> MSVNSIYTDREEIDSEFEDEDFEKEGIATVERAMENNHDLDTALLELNTLRMSMNVTYHEVRIATITALLRRVYHFIATQTLGPKDAVVKVFNQW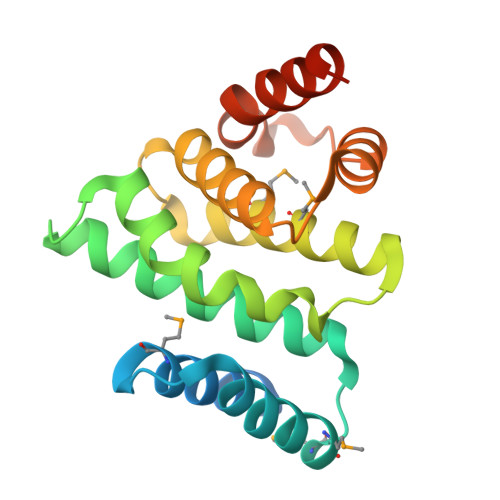GLLFKRQAFDEEEYIDLMNIIMEKIVEQSFDKPDLILFSALVSLYDNDIIEEDVIYKWWDNVSTDPRYDEVKKLTVKWVEWLQNADEESSSEEE>[4x]GSERQILRLKQINIQLATKIQHLE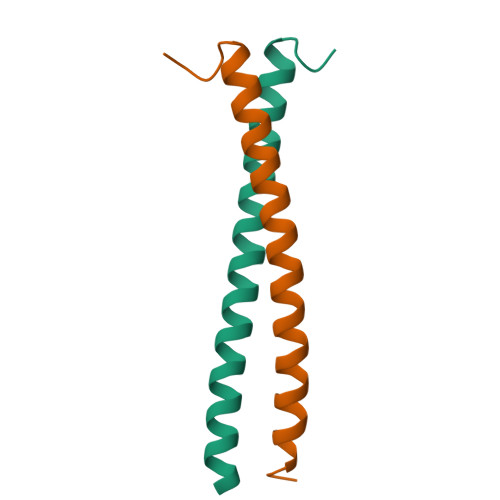FSSSEKEQEIERLNKLLKQNGLLGDVN>[2x]GSH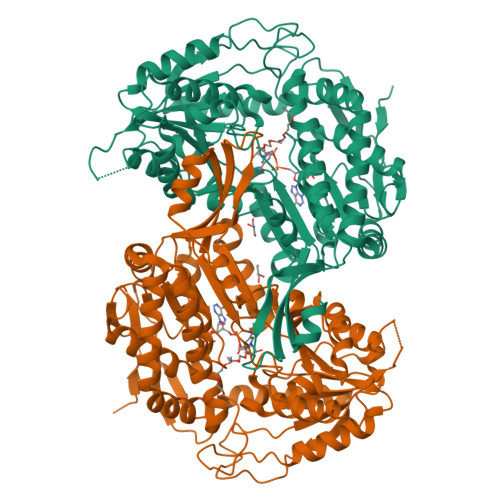MTELLKNHVAGQWIAGTGAGITLTDPVTGVALVRVSSEGLDLARAFSFAREDGGAALRALTYAQRAARLADIVKLLQAKRGDYYAIATANSGTTRNDSAVDIDGGIFTLSYYAKLGASLGEVHALRDGSAESLSKDRSFSAQHVLSPTRGVALFINAFNFPSWGLWEKAAPALLSGVPVIVKPATATAWLTQRMVADVVDAGILPPGALSIICGSSAGLLDQIRSFDVVSFTGSADTAATLRAHPAFVQRGARLNVEADSLNSAILCADATPDTPAFDLFIKEVVREMTVKSGQKATAIRRAFVPEAALEPVLEALKAKLAKITVGNPRNDAVRMGSLVSREQYENVLAGIAALREEAVLAYDSSAVPLIDADANIAACVAPHLFVVNDPDNATLLHDVEVFGPVASVAPYRVTTDTNALPEAHAVALARRGQGSLVASIYSNDDAHLGRLALELADSHGRVHAISPSVQHSQTGHGNVMPMSLHGGPGRAGGGEELGGLRALAFYHRRSAIQAASAAIGTLTQATHWPAA> MAHHHHHHATLLYGKNN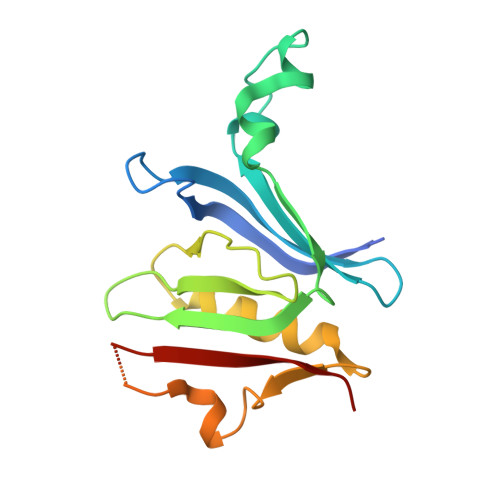VLVQPRDDMEAVPGYLSLHQTADVMTLKWTPNQLMNGSVGDLDYEKSVYWDYAVTIRLEEIVYLHCHQQVDSGGTVVLVSQDGIQRPPFRFPKGGHLLQFLSCLENGLLPHGQLDPPLWSQRGKGKVFPKLRKRSPQGSSESTSSDKEDDEATDYVFRIIYPG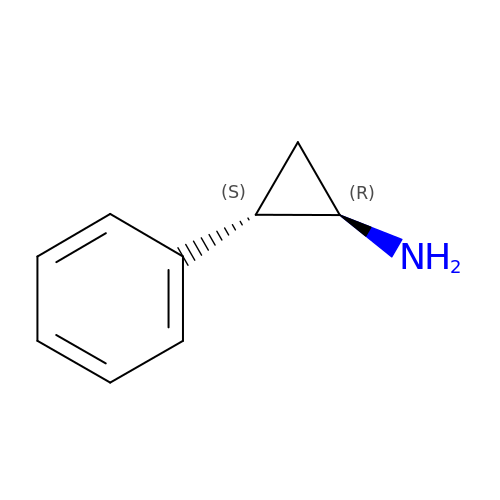(1R,2S)-2-phenylcyclopropanamine | C9 H11 N | AELCINSCMGFISI-DTWKUNHWSA-N>[2x]SGAMYIDCDGIKLNAYLDMPKNNPEKCPLCIIIHGFTGHSEERHIVAVQETLNEIGVATLRADMYGHGKSDGKFEDHTLFKWLTNILAVVDYAKKLDFVTDIYMAGHSQGGLSVMLAAAMERDIIKALIPLSP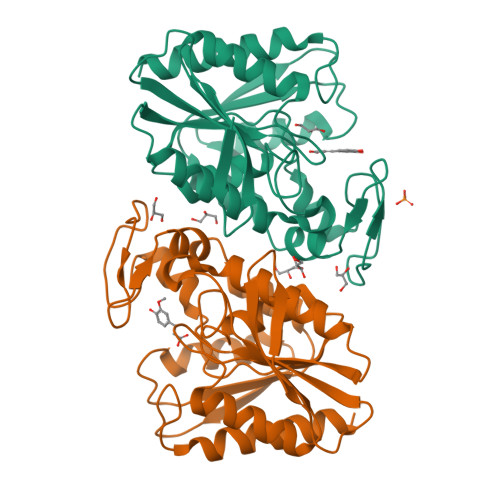AAMIPEIARTGELLGLKFDPENIPDELDAWDGRKLKGNYVRVAQTIRVEDFVDKYTKPVLIVHGDQDEAVPYEASVAFSKQYKNCKLVTIPGDTHCYDHHLELVTEAVKEFMLEQIAK> RRRRRSWY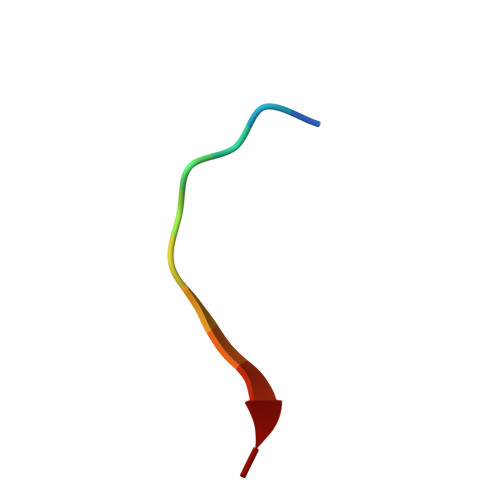FDG> MSELITENMHMKLYMEGTVNNHHFKCTSEGEG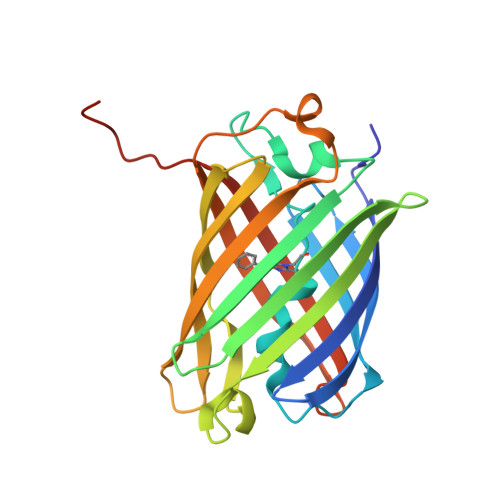KPYEGTQTQRIKVVEGGPLPFAFDILATSFMYGSHTFINHTQGIPDFWKQSFPEGFTWERVTTYEDGGVLTATQDTSLQDGCLIYNVKIRGVNFPSNGPVMQKKTLGWEAHTEMLYPADGGLEGRADLALKLVGGGHLICNFKTTYRSKKPAKNLKMPGVYYVDYRLERIKEADKETYVEQHEVAVARYCDLPSKLGHKLN>[2x]MNPAAEAEFNILLATDSYKVTHYKQYPPNTSKVYSYFECREKKTENSKLRKVKYEETVFYGLQYILNKYLKGKVVTKEKIQEAKDVYKEHFQDDVFNEKGWNYILEKYDGHLPIEIKAVPEG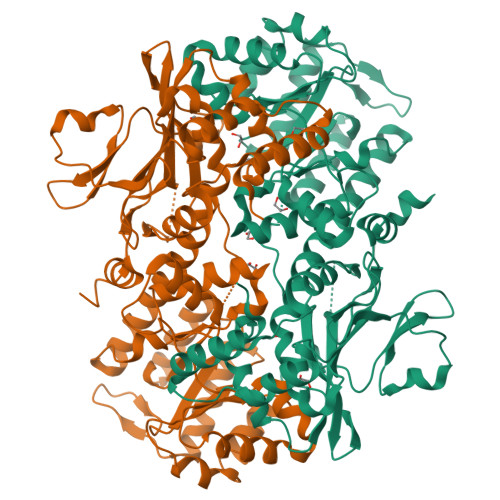FVIPRGNVLFTVENTDPECYWLTNWIETILVQSWYPITVATNYREQKKILAKYLLETSGNLDGLEYKLHDFGYRGVSSQETAGIGASAHLVNFKGTDTVAGLALIKKYYGTKDPVPGYSVPAAEHSTITAWGKDHEKDAFEHIVTQFSSVPVSVVSDSYDIYNACEKIWGEDLRHLIVSRSTQAPLIIRPDSGNPLDTVLKVLEILGKKFPVTENSKGYKLLPPYLRVIQGDGVDINTLQEIVEGMKQKMWSIENIAFGSGGGLLQKLTRDLLNCSFKCSYVVTNGLGINVFKDPVADPNKRSKKGRLSLHRTPAGNFVTLEEGKGDLEEYGQDLLHTVFKNGKVTKSYSFDEIRKNAQLNIELEAAHHLEHHHHHHHH>[2x]MASDVTVNVSAEKQVIRGFGGMNHPAWAGDLTAAQRETAFGNGQNQLGFSILRIHVDENRNNWYKEVETAKSAVKHGAIVFASPWNPPSDMVETFNRNGDTSAKRLKYNKYAAYAQHLNDFVTFMKNNGVNLYAISVQNEPDYAHEWTWWTPQEILRFMRENAGSINARVIAPESFQYLKNLSDPILNDPQALANMDILGTHLYGTQVSQFPYPLFKQKGAGKD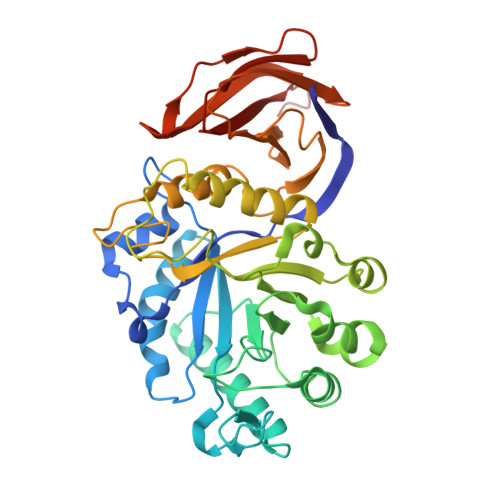LWMTEVYYPNSDTNSADRWPEALDVSQHIHNAMVEGDFQAYVWWYIRRSYGPMKEDGTISKRGYNMAHFSKFVRPGYVRIDATKNPNANVYVSAYKGDNKVVIVAINKSNTGVNQNFVLQNGSASNVSRWITSSSSNLQPGTNLTVSGNHFWAHLPAQSVTTFVVNRLEHHHHHHHH> DTLDEAERQWKAEFHRWSSYM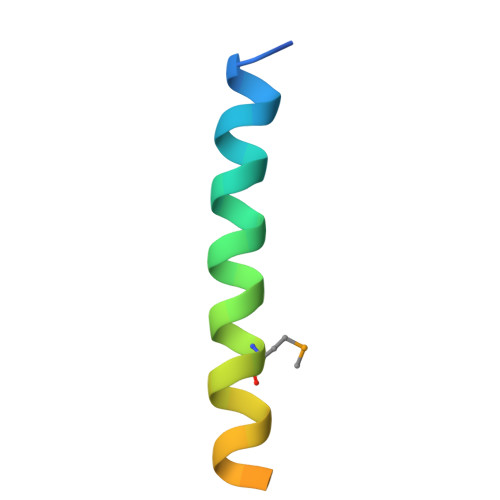VHWKNQFDHYSKQDRCSDL> VPPALHLVDPQIQLTITRADPKVYPIILRLGSNLSLSMARRNLDSLEARAFQSTPI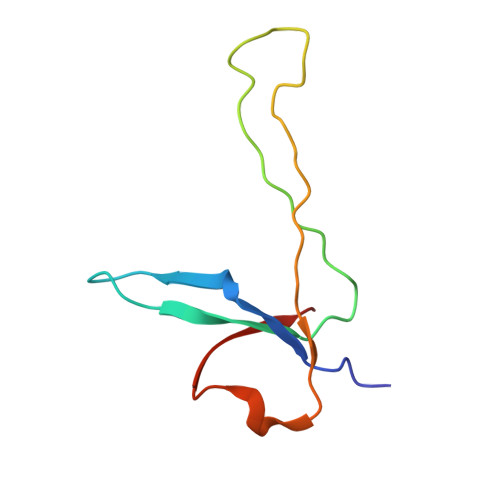VVQMTKLATTEELPDEFVVVTAK> GQAAADRRTVEKTWALMDAVVRLCQNPKLQL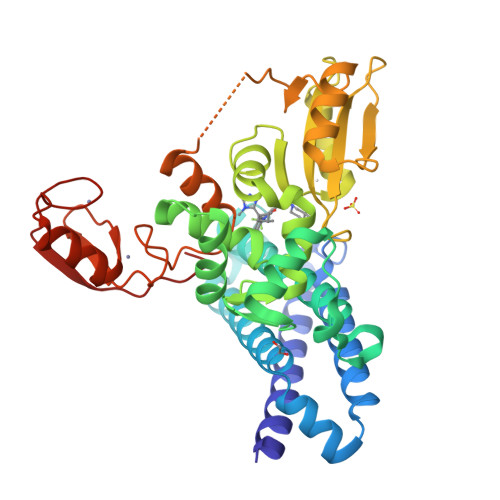KNSPPYILDILPDTYQHLRLILSKYDDNQKLAQLSENEYFKIYIDSLMKKSKRAIRLFKEGKERMYEEQSQDRRNLTKLSLIFSHMLAEIKAIFPNGQFQGDNFRITKADAAEFWRKFFGDKTIVPWKVFRQCLHEVHQISSGLEAMALKSTIDLTCNDYISVFEFDIFTRLFQPWGSILRNWNFLAVTHPGYMAFLTYDEVKARLQKYSTKPGSYIFRLSCTRLGQWAIGYVTGDGNILQTIPHNKPLFQALIDGSAEGFYLYPDGRSYNPDLTGLCEPTPHDHIKVTQEQFELYCEMGSTFQLCKICAENDKDVKIEPCGHLMCTSCLTAWQESDGQGCPFCRCEIKGTEPIIVDPFD> NEAISVEKSIQEQKLNGYGVGSLIKFPVSS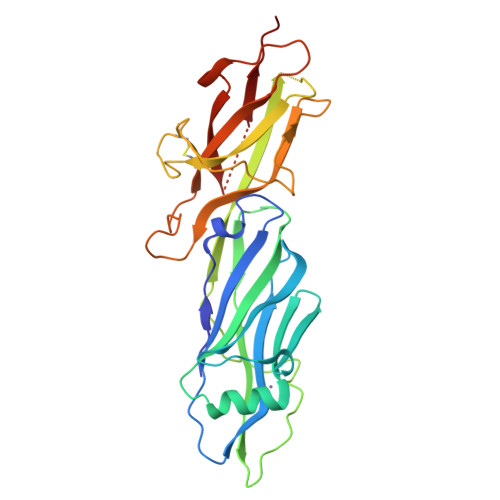TAPTLDAKSFYKYFQLRDTLDDRLTAVTATEVSLEGTTLDPTDYKVDTKGQTVTVTFTAEGLKRIKAAPGKKVSAVFQGKVTEARNGAITNRAQVISDTVYAEQPPTPEEPPANPENPPTSNEVTSRWGDLLIKKVDNHQQGQDKAGLQGAQFQLYKAKNAYAGTCTKDKEGDPIAINGETTLTTDAQGAINVKGLFISDSIDGANRDNQKDATARCYVLVETKAPAGYVLPAGDGAVTPVKIEVGAVTTDNVTIENTKQ> MPGLSCRFYQHKFPEVEDVVMVNVRSIAEMGAYVSLLE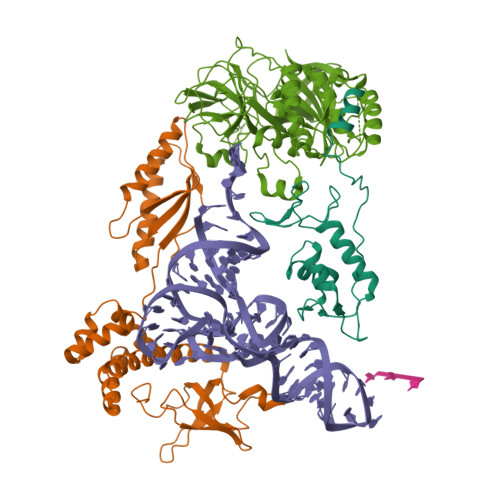YNNIEGMILLSELSRRRIRSINKLIRIGRNECVVVIRVDKEKGYIDLSKRRVSPEEAIKCEDKFTKSKTVYSILRHVAEVLEYTKDEQLESLFQRTAWVFDDKYKRPGYGAYDAFKHAVSDPSILDSLDLNEDEREVLINNINRRLTPQAVKIRADIEVACYGYEGIDAVKEALRAGLNCSTENMPIKINLIAPPRYVMTTTTLERTEGLSVLSQAMAVIKEKIEEKRGVFNVQMEPKVVTDTDETELARQMERLERENAEVDGDDDAEEMEAKAED;> MSGDEMIFDPTMSKKKKKKKKPFMLDEEGDTQTEETQPSETKEVEPEPTEDKDLEADEEDTRKKDASDDLDDLNFFNQKKKKKKTKKIFDIDEAEEGVKDLKIESDVQEPTEPEDDLDIMLGNKKKKKKNVKFPDEDEILEKDEALEDEDNKKDDGISFSNQTGPAWAGSERDYTYEELLNRVFNIMREKNPDMVAGEKRKFVMKPPQVVRVGTKKTSFVNFTDICKLLHRQPKHLLAFLLAELGTSGSIDGNNQLVIKGRFQQKQIENVLRRYIKEYVTCHTCRSPDTILQKDTRLYFLQCETCHSRCSVASIKTGFQAVTGKRAQLRAKAN;> MAGGEAGVTLGQPHLSRQDLTTLDVTKLTPLSHEVISRQATINIGTIGHVAHGKSTVVKAISGVHTVRFKNELERNITIKLGYANAKIYKLDDPSCPRPECYRSCGSSTPDEFPTDIPGTKGNFKLVRHVSFVDCPGHDILMATMLNGAAVMDAALLLIAGNESCPQPQTSEHLAAIEIMKLKHILILQNKIDLVKESQAKEQYEQILAFVQGTVAEGAPIIPISAQLKYNIEVVCEYIVKKIPVPPRDFTSEPRLIVIRSFDVNKPGCEVDDLKGGVAGGSILKGVLKVGQEIEVRPGIVSKDSEGKLMCKPIFSKIVSLFAEHNDLQYAAPGGLIGVGTKIDPTLCRADRMVGQVLGAVGALPEIFTELEISYFLLRRLLGVRTEGDKKAAKVQKLSKNEVLMVNIGSLSTGGRVSAVKADLGKIVLTNPVCTEVGEKIALSRRVEKHWRLIGWGQIRRGVTIKPTVDDD> AASLYEK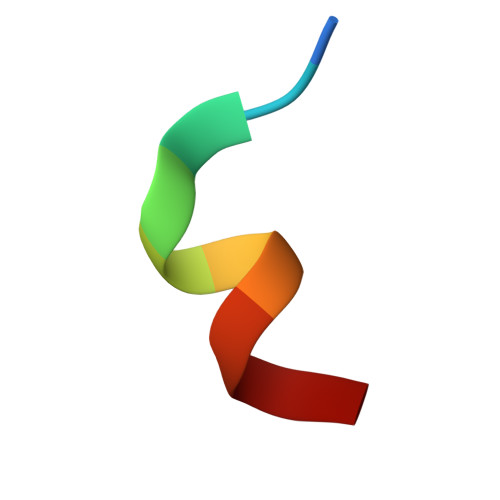KAA Lytic transglycosylases (LTs) degrade peptidoglycan (PG) to produce N-acetylglucosamine (GlcNAc)−1,6-anhydro-N-acetylmuramic acid (MurNAc)-peptide (G-anhM-peptide), a key cytotoxic elicitor of harmful innate immune responses. The crystal structure of the outer membrane lipoprotein LtgA, a homolog of Slt70 that belongs to family 1A of GH family 23 from the pathogenic Neisseria species, was previously determined at a resolution of 1.4 Å.. Briefly, LtgA is a highly alpha-superhelical structure consisting of 37 alpha helices. The active site of LtgA is formed by ten alpha helices (α 28, 29, 30, 31, 32, 33, 34, 35, 36, 37), with a six-alphahelix bundle (α 29, 30, 31, 32, 33, 34) constituting the core of the active site that firmly secures the glycan chain.

In the course of monitoring the LtgA reaction in the crystalline state, we captured a native version of LtgA with a distinctly disordered alpha helix 30. This represents a newly identified conformational state of LtgA whereby alpha helix 30 transitions from an ordered to a disordered state. Interestingly, this disorder of alpha helix 30 did not affect the overall structural integrity of the active site because all the other helices making up the catalytic domain remained intact. Moreover, LtgA was already shown to be active in the crystalline state in our previous studies, although the molecular details of alpha helix 30 interactions with the ligand was not addressed (Williams et al., 2018). In this study, we identified a variant of LtgA with a disordered active site alpha helix 30, which is important for PG binding and for the catalytic mechanism of LtgA. When LtgA, missing the alpha helix 30 motif, was expressed from an ectopic locus in N. meningitidis (at an elevated level compared to wild type), bacterial growth, cell division and daughter cell separation were disrupted, compromising the integrity of the cell wall and PG composition, and diminishing bacterial fitness or virulence in a mouse infection model. In our ΔltgAltgAΔ30 strain, we observed significant defects in growth, cell division, cell separation, cell membrane irregularities, and fibrous and membranous extra cellular material, which were noticeably absent in the wild type, ΔltgA, and the ΔltgAltgA strains. However, the PG of the ΔltgAltgAΔ30 strain was found to be markedly hyperacetylated when compared to that of the other strains, with a 102% increase in the amount of acetylated GlcNAc-anhMurNAc-tetrapeptide (GM*4), a 39% increase in acetylated GlcNAc-anhMurNAc-tetrapeptide crosslinked with GlcNAc-MurNAc-tetrapeptide (GM*4-GM4), and a 46% increase in doubly acetylated di-GlcNAc-anhMurNAc-tetrapeptide (GM*4 GM*4). LtgA enhances the activity of Ape1 and an impaired LtgA results in a dysfunctional Ape1, and appears to poison the cell wall machinery with devastating effects toward the survival of Neisseria in the host.

> MYLPSMKHSLPLLAALVLAACSSTNTLPAGKTPADNIETADLSASVPTRPAEPERKTLADYGGYPSALDAVKQKNDAAVAAYLENAGDSAMAENVRNEWLKSLGARRQWTLFAQEYAKLEPAGRAQEVECYADSSRNDYTRAAELVKNTGKLPSGCTKLLEQAAASGLLDGNDAWRRVRGLLAGRQTTDARNLAAALGSPFDGGTQGSREYALLNVIGKEARKSPNAAALLSEMESGLSLEQRSFAWGVLGHYQSQNLNVPAALDYYGKVADRRQLTDDQIEWYARAALRARRWDELASVISHMPEKLQKSPTWLYWLARSRAATGNTQEAEKLYKQAAATGRNFYAVLAGEELGRKIDTRNNVPDAGKNSVRRMAEDGAVKRALVLFQNSQSAGDAKMRRQAQAEWRFATRGFDEDKLLTAAQTAFDHGFYDMAVNSAERTDRKLNYTLRYISPFKDTVIRHAQNVNVDPAWVYGLIRQESRFVIGAQSRVGAQGLMQVMPATAREIAGKIGMDAAQLYTADGNIRMGTWYMADTKRRLQNNEVLATAGYNAGPGRARRWQADTPLEGAVYAETIPFSETRDYVKKVMANAAYYAALFGAPHIPLKQRMGIVPAR> MIPPRIVPWRDFAELEELKLWFYPKSKGTIEDKRQRAVQRVQSYRLKGSQYLPHVVDSTAQITCAVLLDEKEACLGVHQDSIPIRLSYVMALIRFVNGLLDPTQQSQFAIPLHTLAAKIGLPSWFVDLRHWGTHERDLPGLEMLRWAANEALSWLYDHYWNDEELEDDRDDDDDDDDTGYGYRRNDKLEKYMESLTKTLDKWKRLRNEFLE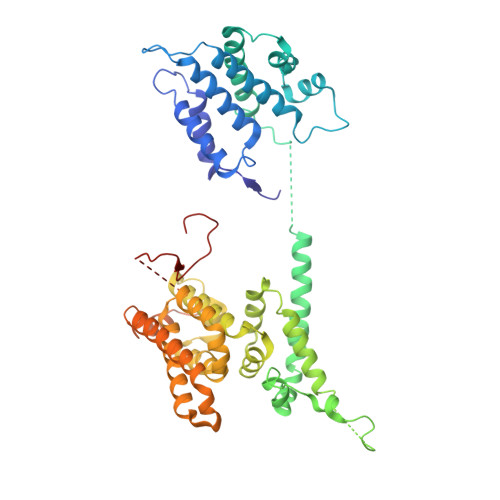YKWVWENANDSLITSSNFSGDNLVNYDAEKRKSSHASSSETMIRENLRQWQELWKLSIYHNVVLEKFFNNYDPLLLKVLMLNLNNFDWKVIEWVARNYRTQQDDSNITTILKRKFNAWKELQKRLLDVIINNLNNKNFKNKWQNWEKLIDENASYLILYFCQSMLAKLETEKITGNSWRNKKRRKQIDSTVEIEAKLKENIDNLSLRFNEGEIKLYDFIPAEKDSVPLKKEVSPALKADTNDILGDLASLKQRMSSFGTVGKKNKQEENRATPVKNWSRVQNWKPKPFGVL>TNLISVNSRSYRLSSAPTIVICVDGCEQEYINQAIQAGQAPFLAELTGFGTVLTGDCVVPSFTNPNNLSIVTGAPPSVHGICGNFFFDQETQEEVLMNDAKYLRAPTILAEMAKAGQLVAVVTAKDKLRNLLGHQLKGICFSAEKADQVNLEEHGVENILARVGMPVPSVYSADLSEFVFAAGLSLLTNERPDFMYLSTTDYVQHKHAPGTPEANAFYAMMDSYFKRYHEQGAIVAITADHGMNAKTDAIGRPNILFLQDLLDAQYGAQRTR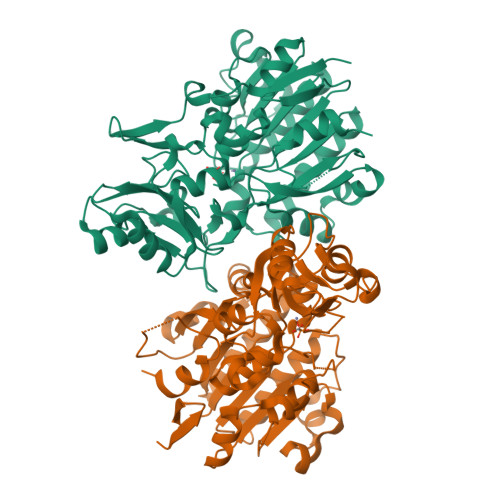VLLPITDPYVVHHGALGSYATVYLRDAVPQRDAIDFLAGIAGVEAVLTRSQACQRFELPEDRIGDLVVLGERLTVLGSAADKHDLSGLTVPLRSHGGVSEQKVPLIFNRKLVGLDSPGRLRNFDIIDLALNHLA[4x]> MFSAGHKIKGTVVLMPKNELEVNPDGSAVDNLNAFLGRSVSLQLISATKADAHGKGKVGKDTFLEGINTSLPTLGAGESAFNIHFEWDGSMGIPGAFYIKNYMQVEFFLKSLTLEAISNQGTIRFVCNSWVYNTKLYKSVRIFFANHTYVPSETPAPLVEYREEELKSLRGNGTGERKEYDRIYDYDVYNDLGNPDKSEKLARPVLGGSSTFPYPRRGRTGRGPTVTDPNTEKQGEVFYVPRDENLGHLKSKDALEIGTKSLSQIVQPAFESAFDLKSTPIEFHSFQDVHDLYEGGIKLPRDVISTIIPLPVIKELYRTDGQHILKFPQPHVVQVSQSAWMTDEEFAREMIAGVNPCVIRGLEEFPPKSNLDPAIYGDQSSKITADSLDLDGYTMDEALGSRRLFMLDYHDIFMPYVRQINQLNSAKTYATRTILFLREDGTLKPVAIELSLPHSAGDLSAAVSQVVLPAKEGVESTIWLLAKAYVIVNDSCYHQLMSHWLNTHAAMEPFVIATHRHLSVLHPIYKLLTPHYRNNMNINALARQSLINANGIVETTFLPSKYSVEMSSAVYKNWVFTDQALPADLIKRGVAIKDPSTPHG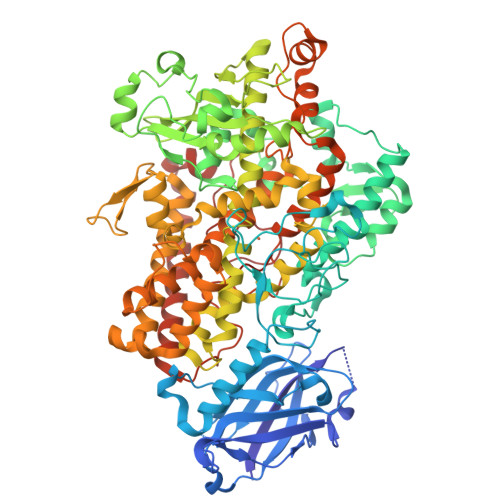VRLLIEDYPYAADGLEIWAAIKTWVQEYVPLYYARDDDVKNDSELQHWWKEAVEKGHGDLKDKPWWPKLQTLEDLVEVCLIIIWIASALHAAVNFGQYPYGGLIMNRPTASRRLLPEKGTPEYEEMINNHEKAYLRTITSKLPTLISLSVIEILSTHASDEVYLGQRDNPHWTSDSKALQAFQKFGNKLKEIEEKLVRRNNDPSLQGNRLGPVQLPYTLLYPSSEEGLTFRGIPNSISI> MERYENLFAQLNDRREGAFVPFVTLGDPGIEQSLKIIDTLIDAGADALELGVPFSDPLADGPTIQNANLRAFAAGVTPAQCFEMLAIIREKHPTIPIGLLMYANLVFNNGIDAFYARCEQVGVDSVLVADVPVEESAPFRQAALRHNIAPIFICPPNADDDLLRQVASYGRGYTYLLSRSGVTGAENRGALPLHHLIEKLKEYHAAPALQGFGISSPEQVSAAVRAGAAGAISGSAIVKIIEKNLASPKQMLAELRSFVSAMKAASRA;> MTTLLNPYFGEFGGMYVPQILMPALNQLEEAFVSAQKDPEFQAQFADLLKNYAGRPTALTKCQNITAGTRTTLYLKREDLLHGGAHKTNQVLGQALLAKRMGKSEIIAETGAGQHGVASALASALLGLKCRIYMGAKDVERQSPNVFRMRLMGAEVIPVHSGSATLKDACNEALRDWSGSYETAHYMLGTAAGPHPYPTIVREFQRMIGEETKAQILDKEGRLPDAV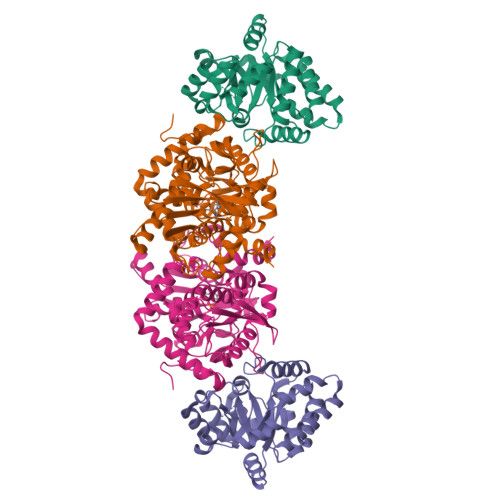IACVGGGSNAIGMFADFINDTSVGLIGVEPGGHGIETGEHGAPLKHGRVGIYFGMKAPMMQTADGQIEESYSISAGLDFPSVGPQHAYLNSIGRADYVSITDDEALEAFKTLCRHEGIIPALESSHALAHALKMMREQPEKEQLLVVNLSGRGDKDIFTVHDILKARGEI Here, we reveal the extended and contracted atomic structures of an intact contractile-tailed phage (φCD508) that binds to and penetrates the protective S-layer of the Gram-positive human pathogen Clostridioides difficile. The virion can be divided into five distinct regions: the head, neck, tail, baseplate, and needle. Structures of purified φCD508 virions in both extended and contracted conformations were determined by single-particle EM of frozen-hydrated samples; the resolution ranged from 2.6 to 4.0 Å for the extended phage, and 2.9 to 4.2 Å for the contracted form.

At the base of the capsid sits a unique opening, centered on what would be a fivefold symmetry axis in a complete icosahedron; it is made up of 12 copies of portal protein gp45, forming an opening through which DNA is ejected from the capsid. Thus, there is a 5–12-fold symmetry mismatch between the capsid and the portal.

>[12x]MGIISYVKKLFKRPAGEIMRMSSGNIGVYKLDDSRVDYELARELYQNKNANYKLGSSFVRPIVNSTTGFMGVPHFQIEDEEAQYILDEFVLDNTSKMLKTHTDSLKQGDCYIWITREERENPLYPDKKVRLIYNFISPEEVKEIILDPTTKEPIAYILESQNEWTDLGENKRKAKVKQIITAESRFVEVEGDKIEGLEEGETPNVWGFIPIIHFKNEADETLKYGQSDIEPIEPLLKAYHDVMLHALKGSKMHSTPKLKLKLTDVASFLAHNFGVEDPVKFAKEGGKINLDGHEILFLNKDEEAEFVEVKSAIGDAKELLKLLFYCIVDVSETPEFIFGVHTPSALASVKEQMPIMVNKIRRKREQFTNSWQLLARMVLIMSSNSSGMKYSSYDVTIGWDEVNPRDDKELAETLEKVCCALDKALEGGFISEESTVNFLAQYIDTMSNYISDDPEREGEREKIIKTKMLKYRLDDSQGLNDESNEIEKEINKIKDNNGNG Here, we characterized Atu1419 as a transcriptional repressor of its own repression in addition to two other genes (atu1418 and atu1420). The structures revealed Atu1419 to be a member of the VanR group of the FadR C-terminal domain (FCD; Pfam PF07729) subfamily of the large GntR superfamily of transcriptional factors (>93 135 members in Pfam database). Like FadR, Atu1419 possesses a characteristic molecular architecture, composed of a conserved N-terminal DNA binding domain containing the wHTH motif and a C-terminal effector binding/oligomerization domain. We identified the short palindromic region composed of 10 base pairs and a degenerated palindrome bound to Atu1419 and the N5,N10-methylenetetrahydrofolate (MEF) as the effector molecule disrupting Atu1419-DNA interaction, allowing the expression of the second part of the HCA degradation pathway.

The structures of two palindromic DNA-Atu1419 complexes solved at 2.79 Å resolution (P6422 space group) and 2.05 Å resolution (C2221 space group) present a distinct neighboring crystal packing with an asymmetric unit containing a monomer bound to a single DNA strand and a dimer bound to the 10-mer palindromic DNA, respectively. Nonetheless, a tetramer, where dimers AB and CD bind each to a DNA palindrome, was reconstituted by crystal symmetries in line with the conservation of Atu1419 tetramer in solution upon DNA binding. The three monomers of the asymmetric units (one in P6422 and two in C2221) are similar with an average RMSD value of 1 Å for all Cα atoms making almost identical interactions with DNA, although the positions of the DNA binding domains within the dimers between the two crystal structures do not completely overlap. Each monomer recognizes a half-site DNA with helices α2 and α3 of the HTH motif making nine polar interactions with both strands in the major groove of the DNA. All Atu1419-DNA subunits contain a bound Zn2+ ion at the same position as that observed in both Atu1419–citrate complexes. In contrast to the protein-DNA complex in C2221 space group, which crystallized in MES buffer, the P6422 protein–DNA complex reveals a bound citrate in the effector binding pocket. This citrate adopts the orientation B described in both Atu1419-citrate complexes, except for molecule A (orientation A) in the P212121 structure. Because both tetrameric Atu1419-DNA structures are similar, the presence of the bound citrate in orientation B in all subunits of one DNA complex has clearly no effect on Atu1419 for DNA binding and DNA release, in agreement with EMSA and promoter activity. Thus, Atu1419 is a tetramer in its apo form, upon DNA binding or effector binding suggesting that this quaternary structure is the biologically active form. Both crystal structures of Atu1419 in complex with DNA revealed that each dimer of Atu1419 within the tetramer can bind a palindromic site of 10 bp, separated by approximately 10 nm.

> MRQVDAATHGGRAVIELREKILSGELPGGMRLFEVSTAELLDISRTPVREALSRLTEEGLLNRLPGGGFVVRRFGFADVVDAIEVRGVMEGTAARLAAERGVSKVALEEIDATVQQLDLCFGDRVDDVDFDGYAALNRIFHHQLAALCGSEMIRREVERASSLPFASPSAFLPDKANIGAFRRSLRGAQEQHKAIVAAIVAREGARAEAVAREHSRTARTNLEYMIREAPELIAQVPGLALISDHHHHHH> MSFLFSSRSSKTFKPKKNIPEGSHQYELLKHAEATLGSGNLRQ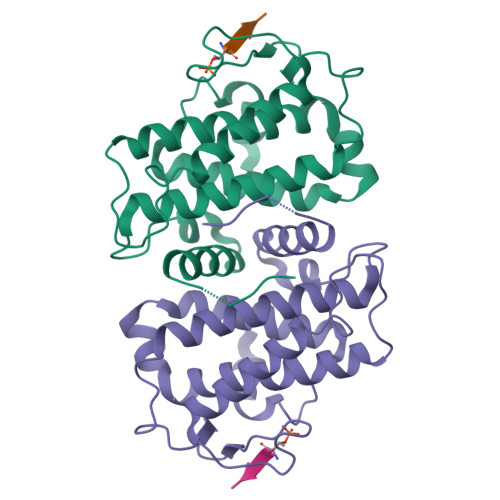AVMLPEGEDLNEWIAVNTVDFFNQINMLYGTITEFCTEASCPVMSAGPRYEYHWADGTNIKKPIKCSAPKYIDYLMTWVQDQLDDETLFPSKIGVPFPKNFMSVAKTILKRLFRVYAHIYHQHFDSVMQLQEEAHLNTSFKHFIFFVQEFNLIDRRELAPLQELIEKLGSKDR;> DDTLPSQLGTMVINAED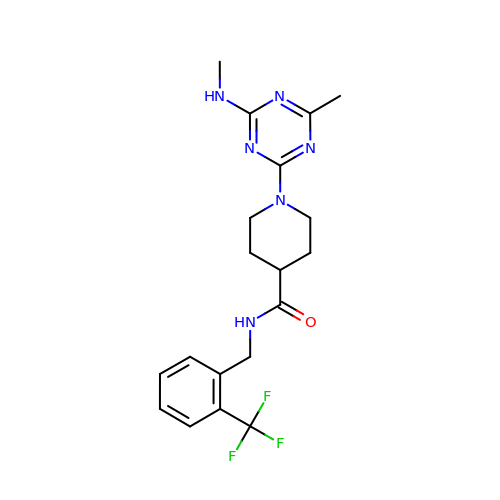1-[4-methyl-6-(methylamino)-1,3,5-triazin-2-yl]-N-[2-(trifluoromethyl)benzyl]piperidine-4-carboxamide | C19 H23 F3 N6 O | BUWQYHYHSQTERY-UHFFFAOYSA-N>[2x]MKKRAIQKIISSIVSLAVLTSVPVMQKPSVLAASSDSTSASKTDFFSSFEKSDLQLTWTNTVETDANGKKMSSGIDGNVKRDLILGDITDKVVQVTASANNPPNEIDSKLIDGDPTTKWLAFEPTANIVLKLAEPVAVVKYALTSANDAKGRDPKNWTLYGSLDGTNWTAVDTREGEDFKDRFQRNMYDLKNTTKYLYYKLDITKNAGDSITQLAEISLSDGIEVPAPPPGDMKSLIGKGPTSSYTAKTNVGWTGLGALNYSGTHLSDGRAYSYNKLYDVDILVTPATELSYFIAPEFTDKNHNDYSSTYVSVDLAFSDGTYLHDLKAVDQYGVGLNPKDQGDSKYLYVNQWNTIKSTIGSVAAGKTIKRILVAYDNPKGPGAFRGSIDDIKIDGKPVQKAFGSPIDYVNILRGTQSNGSFSRGNNFPAVAIPHGFNFWTPTTNAGSSWIYQYHESNSVNNLPQIQAFSVSHEPSPWMGDRQTFQVMPSASTAATPNANRDSRALEFNHANEIAQPHYYSVKFENGIRTEMTPTDHAAMFKFTFTGATSNLIFDNVNNNGGLTIDAKSGEITGYSDVKSGLSTGATRLFVYAAFDKPVIKSGKLTGESRNNVTGYVRFDTSKDEDKVVTMKIATSLISVEQAKKNLEQEIGLNDTFEGLKEKAKTEWN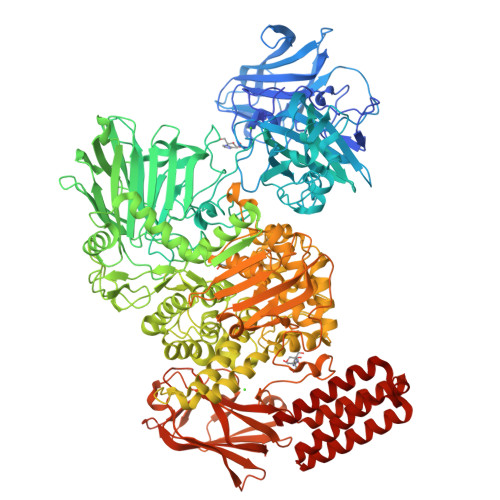KKLGIIEVEGASEDQLVTLYSNLYRLFLYPNSAFENVGTTTDPVYKYASPYSAATGQDTATTTGAKIVDGKTYVNNGFWDTYRTAWPAYSLLTPTFAGELIDGFVQQYRDGGWIARWSSPGFANLMPGTSSDVAFADAYLKGVTNFDVQSFYQSAIRNAEAVSPNAGTGRKGLTTSIFDGYTNTSTGEGLAWAMDGYINDFGIANLAKALKEKGDKSDPYYANYAADYQYFLNRAQNYVHMFNPSIEFFNGRTANGAWRSTPDNFNPAVWGSDYTETNGWNMAFHVPQDGQGLANLYGGKEGLATKLDQFFSTSETGLFPGSYGGTIHEMREARDVRMGMYGHSNQPSHHIAYMYDYAGQPWKTQEKVREALNRLYIGSAIGQGYSGDEDNGEMSAWYILSAMGFYPLKMGTPEYAIGAPLFKKATIHLENGKSIVINAPNNSKENKYVQSMKVNGKAYAKTSILHADIANGAVIDFEMGSKPSKWGSGDQDILQSITPGSTDGTSLSPLPLRDVTDRLIAAEKGAVTVSDEGNGQLLFDNTSNTQLSMKSKTPSIVYQFKEGKQNVKMYTLTSSKASQNEDPKSWVLKGSNDGKSWSVLDQRKNETFQWRQYTRAFTIQHPGKYSQYKLEITENAGAEVTTLAELELLGYDDVTNSYQAVYELMEQFKQSKDLTGPMAVQLNNSLTTSLDHFKKDHKDQAIKHLEDFLKHLNNKGLQDRISSKAKGVLSADANQLIVLLARD>GSHMASMHTVLQIGAGGVGSVVAHKMGMNRDVFKNIILASRSLDKCYAIKESMLKKGLGEIGVEQVDADDTQALVALIQKYKPKVVINVALPYQDLTIMQACLETKTHYIDTANYEHPDLAKFEYKEQWAFDRAYKEARILGVLGAGFDPGVTNAYVAHAQRHHFDTIHTLDILDCNAGDHKRPFATNFNPEINLREVSSKGRYYENGKWIETKPLEIKQVWAYPQIGEMDSYLLYHEELESLVKNIKGLRRARFFMTFSQNYLTHMKCLENVGMLGIKEIEHQGVKIVPIQFLKTLLPDPATLAKDTTGKTNIGCYMTGIKNNQDKTLYIYNVCDHKKCY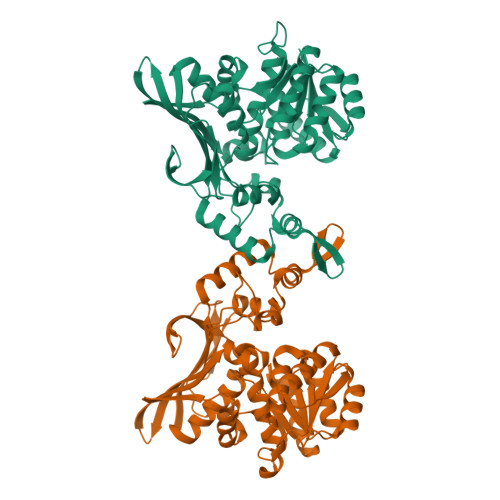EEVGSQAISYTTGVPAMCAAKMICNDTWSADHFRAGVFNIEELNTDPFMEELIKQGLPYEVIER[4x]2,3-DEOXY-3-FLUORO-5-O-TRITYLURIDINE | C28 H25 F N2 O4 | 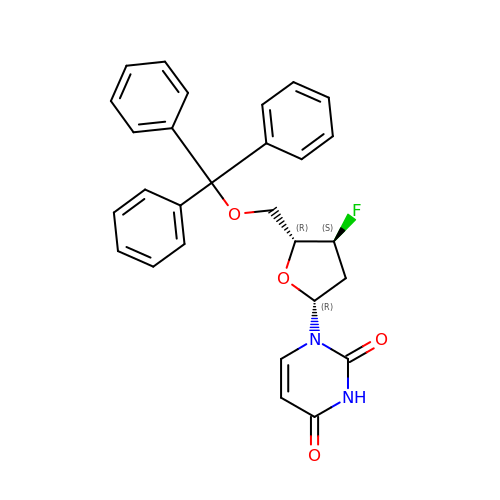GJNIPWYJQUGERM-BFLUCZKCSA-N> MDDIETIEKYGRDETYIFLADSAKRDTAAYPTAAEYEVLFNAQFRNVTKFELLEVNIPRTEYLIDSSENTFAYALNQPTNINTWQQEIEGNIRIATITPGDYNLPQLIDEMNNVLQQTANTYGDSVILQVSPVTNPSEISNKIRITASGPFTLLGSTGTIGNTIGFGDPVNTSVASTTGYYSTVPGYSVNYPNGADYVFLSNQGNIGSEAVNEFVGPLPPGDNVSFTPIYTGQTPSQYFIAPSAGV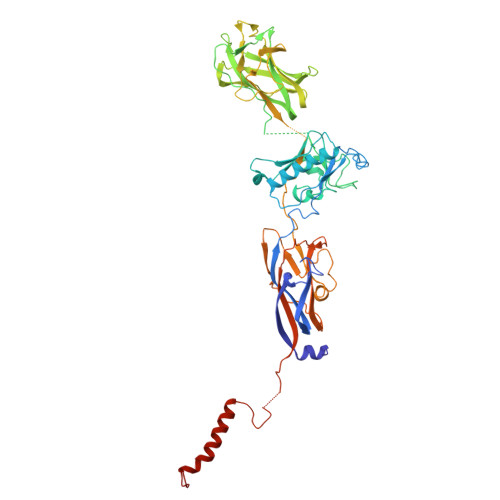PTTVSAYFVDQATAPPGGFVVNYSIIKVSDSSTIATGSLISTNDDLVPSVSSPSVVSANFIQGQQYYIQFTPGSSGSSAGNCTALWYSFPNLPPVSGAYAAINGTLVFPGQYFCTDVSAGAYGNELTSPGIVNITGARYIKIRCKELEQLIYRDRVGEPTTAGIGIVNLIGYGFERSRYDFSSIPVKAFHPIGKLQKLTFRLERPNGTLYDTNGVDNTMLCALTFKVVPNNAVDKTFDGPGKYPAAPGYSGDYIQLQQKRWGEEARATYPTHKSTYNRCRPRTT APP comprises a large extracellular region, a single transmembrane helix and a short cytoplasmic tail containing an NPxY motif (normally referred to as the YENPTY motif). Talins are synaptic scaffold proteins that connect the cytoskeletal machinery to the plasma membrane via binding NPxY motifs in the cytoplasmic tail of integrins. The central adapter that connects integrins to the actin cytoskeleton is the protein talin, which contains 13 helical bundles that behave as force-dependent binary switch domains. Here, we report the crystal structure of an APP/talin1 complex identifying a new way to couple the cytoskeletal machinery to synaptic sites through APP.

Using the design strategy of the β3 (739–749)-talin (209–400) chimera, we generated an APP (754–764)-talin (209–400) chimera, hereafter called the APP-talin chimera. The APP-talin chimera crystals were birefringent flat plates belonging to space group P212121, which diffracted to 2.7 Å. The crystals belong to the space group P212121 with a single copy of the APP-talin1 (F2F3) chimera in the asymmetric unit (AU). In contrast to the β3-integrin-talin chimera, which adopted a homodimeric arrangement in the asymmetric unit mediated by reciprocal F3-NPxY interactions of the two fusion proteins, the APP-talin chimera showed a ‘daisy chain’ style arrangement where each APP tail interacted with the F3 domain of a symmetry-related molecule. The NPTY was well resolved in the density and closer inspection confirmed that the NPxY motif of the APP was binding canonically in the NPxY motif binding site on talin F3. The mainchain density for the APP (754–764) is well defined and the side chains for N759–F764 (including the NPxY motif) could be unambiguously placed. The final model comprises residues 209–400 of talin1 (F2F3), with residues K322 and N323 missing from the loop in F3 that connects β1 and β2. The chemical shift changes upon addition of APP peptide in the NMR data precisely map onto the APP-interacting surface on F3. The crystal structure of the NPxY motif of APP bound to talin identifies the APP cytoplasmic tail as a second attachment site for talin to engage, with the potential to forge similar cytoskeletal connections at the synaptic junction. In this assay, the APP and APP (4A) peptides are fluorescently tagged by covalently coupling a fluorescein-maleimide to a non-native terminal cysteine and titrated with both talin1 and talin2 F2F3 domains. This confirmed that (i) both talin isoforms bind to APP and (ii) the interaction is specific but weak as expected since talin also binds weakly to the NPxY motif of the β-integrin cytoplasmic tail in solution (with Kd in the range of 100–1000 µM).

> GIDPFTQNGYENPTYKF;> PVQLNLLYVQARDDILNGSHPVSFDKACEFAGYQCQIQFGPHNEQKHKPGFLELKDFLPKEYIKQKGERKIFMAHKNCGNMSEIEAKVRYVKLARSLKTYGVSFFLVKEKMKGKNKLVPRLLGITKECVMRVDEKTKEVIQEWSLTNIKRWAASPKSFTLDFGDYQDGYYSVQTTEGEQIAQLIAGYIDIIL[3-(dibutylamino)propyl]phosphonic acid 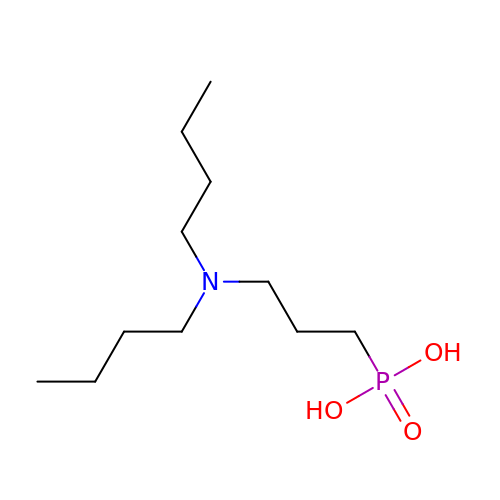| C11 H26 N O3 P | XATRQYYMOIGUKL-UHFFFAOYSA-N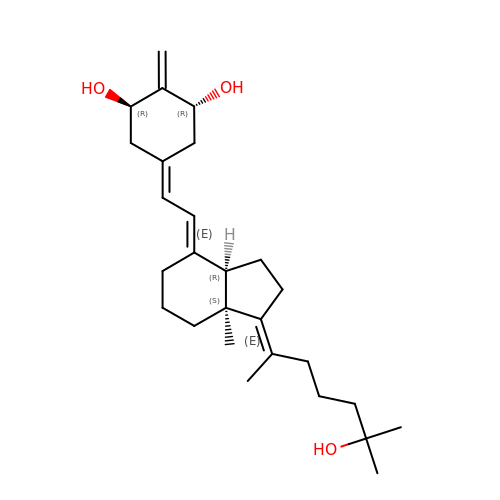(1R,3R,7E,17E)-17-(5-hydroxy-1,5-dimethylhexylidene)-2-methylene-9,10-secoestra-5,7-diene-1,3-diol | C27 H42 O3 | PCPYFQNISYYIPU-QEWVMUDDSA-N> GAMASGKVVKFSYMWTINNFSFCREEMGEVIKSSTFSSGAN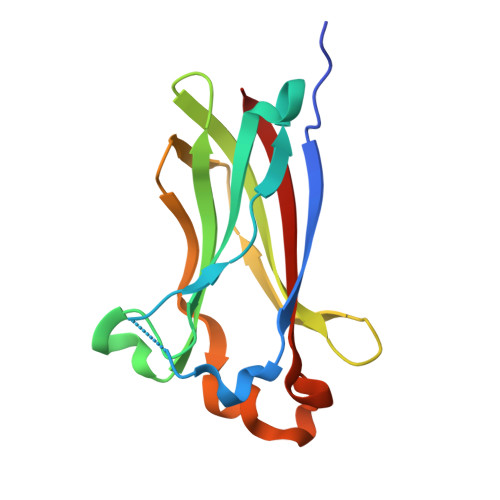DKLKWCLRVNPKGLDEESKDYLSLYLLLVSCPKSEVRAKFKFSILNAKGEETKAMESQRAYRFVQGKDWGFKKFIRRDFLLDEANGLLPDDKLTLFCEVSVVQD> GLECKPRPLHKTCSLFMRNIAPNISRAEIISLCKRYPGFMRVALSEPQPERRFFRRGWVTFDRSVNIKEICWNLQNIRLRECELSPGVNRDLTRRVRNINGITQHKQIVRNDIKLAA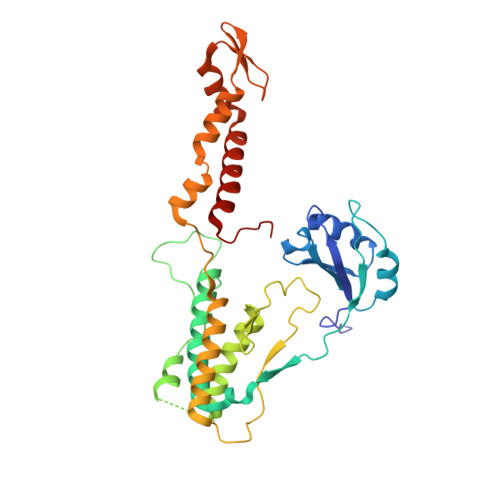KLIHTLDDRTQLWASEPGTPPLPTSLPSQNPILKNITDYLIEEGSGSGSERDEKLIKVLDKLLLYLRIVHSLDYYNTCEYPNEDEMPNRCGIIHVRGPMPPNRISHGEVLEWQKTFEEKLTPLLSVRESLSEEEAQKMGRKDPEQEVEKFVTSNTQELGKDKWLCPLSGKKFKGPEFVRKHIFNKHAEKIEEVKKEVAFFNNFLTDAKRPALPE>GHMPLLSASIVSAPVVTSETYVDIPGLYLDVAKAGIRDGKLQVILNVPTPYATGNNFPGIYFAIATNQGVVADGCFTYSSKVPESTGRMPFTLVATIDVGSGVTFVKGQWKSVRGSAMHIDSYASLSAIWGTAA[10x]

In this study, we evaluate the potential of synthetic fucosylamides as inhibitors of the two lectins LecB (P. aeruginosa) and BC2L-C-Nt (B. cenocepacia). LecB folds as a nine stranded antiparallel β-sandwich with a Greek key motif and two β-sheets composed of four and five strands, respectively. BC2L-C is a hexamer that displays a double sugar specificity: the LecB-like calcium-dependent C-terminal dimeric domain is specific for heptose/mannose, while the N-terminal trimeric domain BC2L-C-Nt is l-fucose-specific and binds histo-blood group oligosaccharides, such as the H-type 1 antigen. LecB from P. aeruginosa binds most compounds of this class in the nM range, whereas BC2L-C-Nt from B. cenocepacia has a more stringent specificity toward the aglycone of this class and additionally only has μM affinity for the best derivatives.

In particular, 1 (SPR KD = 330 μM) displayed an affinity comparable to that of 2. To solve the structure of BC2L-C-Nt in complex with 1 new cocrystallization conditions were found, consisting of 17% Peg10K, 100 mM sodium acetate, and 100 mM Bis-Tris at pH 5.5. The structure could be solved at 2.55 Å in space group H32 with 10 molecules in the asymmetric unit comprising 3 trimers and one protomer along the 3-fold axis where the trimer is obtained by applying symmetry. Electron density is clearly observed for the aglycone in all protomers, while in some protomers one of the two structural waters could not be modeled. The two benzene rings of 1 bind in the narrow cleft of BC2L-C-Nt through hydrophobic and van der Waals interactions. The two aromatic rings of 1 in the complex are not coplanar but form a dihedral angle of about 28°. This orientation allows the distal phenyl ring to burrow into the crevice, while the vicinal ring interacts with Tyr58 in a T-shaped π-stacking. Considering that, both, the benzamide 12 and the naphthylamide 11 have negligible affinity for BC2L-C-Nt, the hydrophobic interaction of the distal phenyl ring of 1 in the deepest section of the binding site may represent a major contribution to the binding affinity of this ligand. In particular, the analysis of the dihedral angle between the amide and the biphenyl group (O–C–CPh–Co-Ph) revealed a rotation of approximately 130°, with values of −160° in the BC2L-C-Nt complex and around −31° in the LecB complex. In BC2L-C-Nt, the binding site is found at the interface between two protomers and is more buried and extended than the site in LecB, which is shallower and solvent exposed.>MRIPLVGKDSIESKDIGFTLIHEHLRVFSEAVRQQWPHLYNEDEEFRNAVNEVKRAMQFGVKTIVDPTVMGLGRDIRFMEKVVKATGINLVAGTGIYIYIDLPFYFLNRSIDEIADLFIHDIKEGIQGTLNKAGFVKIAADEPGITKDVEKVIRAAAIANKETKVPIITHSNAHNNTGLEQQRILTEEGVDPGKILIGHLGDTDNIDYIKKIADKGSFIGLDRYGLDLFLPVDKRNETTLRLIKDGYSDKIMISHDYCCTIDVGTAKPEYKPKLAPRWSITLIFEDTIPFLKRNGVNEEVIATIFKENPKKFFS[4x]

PLLs are natural lactonases endowed with promiscuous phosphotriesterase activity. The catalytic center contained two metal cations coordinated by four histidines, an aspartic acid and a carboxylated lysine residue. A structural analysis of SsoPox, a hyperthermostable counterpart of the PLL family from Sulfolobus solfataricus, has revealed that loop 7 is shorter in SsoPox than in PTEs; linking the active site to the loop 8, which forms a hydrophobic channel that accommodates AHLs aliphatic chain. Indeed, W263 is located at the start of loop 8, involved in the dimer interface of the enzyme and positions the lactone cycle of the substrate onto the bi-metallic catalytic center.

A single mutation of W263 can significantly increase the paraoxonase activity of the enzyme (by 23-fold with the W263F substitution), the oxo-lactonase activity (by 148-fold with the W263T substitution) and the activity toward the poor AHL substrate (3-oxo-C12 AHL; by 55-fold (W263V)). However, whereas detergent-induced flexibility has no effect on the lactonase activity, we isolated variants of W263 that exhibit increased lactonase activities (W263T/V/I). These variants exhibit dramatic improvement of their oxo-lactonase catalytic efficiencies (148-fold for variant W263T), while the activity for the best AHL substrate is compromised (3-oxo-C10 AHL; for the wild-type enzyme). Conversely, the LacSV group dramatically increases oxo-lactonase activity and 3-oxo-C12 AHLase activities, while the phosphotriesterase activity is mildly modulated and 3-oxo-C10 AHLase is decreased. The residues selected in the LacSV group (T, V, I) are overall smaller than those selected in the PteSV group (F, L, M) with the exception of isoleucine (I). Mutations W263V-T therefore yield enlarged active site cavities for the lactone variants. Notably, contrary to the wild-type enzyme, all selected variants (with the exception of W263F) exhibit a substrate inhibition for undecanoic-δ-lactones with KI values ranging between 789 ± 186 µM and 7 400 ± 2 475 µM, respectively, for the W263V and W263M variants. Indeed, all variants exhibit a lower Tm compared to the wild-type enzyme (between 92.0 ± 2.1 °C for SsoPox-W263L to 84.1 ± 1.6 °C for SsoPox-W263V). The analysis of the normalized B-factors of the variants clearly reveal that the substitution W263 is destabilizing (as confirmed by the Tm of the variants), but also that the active site loops of PteSV are significantly more disordered than those of LacSV. PteSV lose their activity before the loss of the global structure (Tm), whereas LacSV do not, and exhibit a similar thermophilicity profile to that of the wild-type enzyme.> MGVLRIGHASLKVMDMDAAVRHYENVLGMKTTMKDKAGNVYLKCWDEWDKYSVILTPSDQAGMNHLAYKVEKEADLEALQQKIEAWGVKTTMLDEGTLPSTGRMLQFKLPSGHEMRLYASKEFVGTDVGNINPDPWPDGLKGAGAHWLDHCLLVCEMNPEAGINTVADNTRFVTECLDFFLTEQVLVGPGGSIQATTFLARTTTPHDIAFVGGPTSGLHHIAFFLDSWHDVLKAADVMAKNKVRIDVAPTRHGITRGETIYFFDPSGNRNETFAGLGYLAQ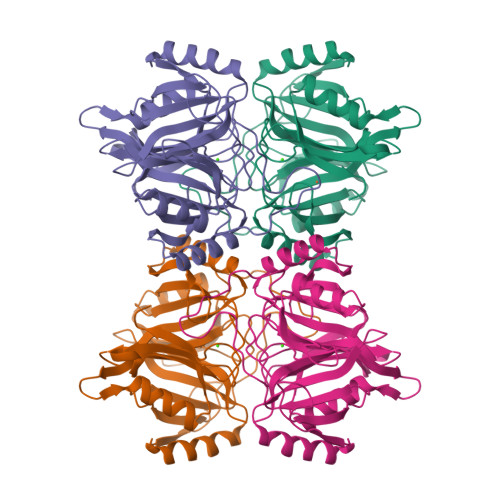RDRPVTTWTEDQ>GAPAAVDWRARGAVTAVKDQGQCGSSWAFSAIGNVECQWFLAGHPLTNLSEQMLVSCDKTDSGCSGGLMNNAFEWIVQENNGAVYTEDSYPYASGEGISPPCTTSGHTVGATITGHVELPQDEAQIAAWLAVNGPVAVAVDASSWMTYTGGVMTSCVSEQLDHGVLLVGYNDSAAVPYWIIKNSWTTQ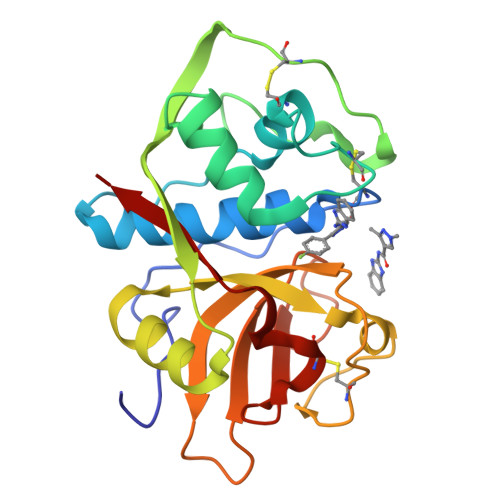WGEEGYIRIAKGSNQCLVKEEASSAVVG[5x]>[4x]SIKSEFAEGAAVFVEGVAVFLTMMAAFQNGDKEAVAQYLARGASLYTRHEELLNRLLQKLRREGNKEAVTLMNEFTATFQTGKSLANALIAAFKNGDDDSFESYLQAIWKVIAK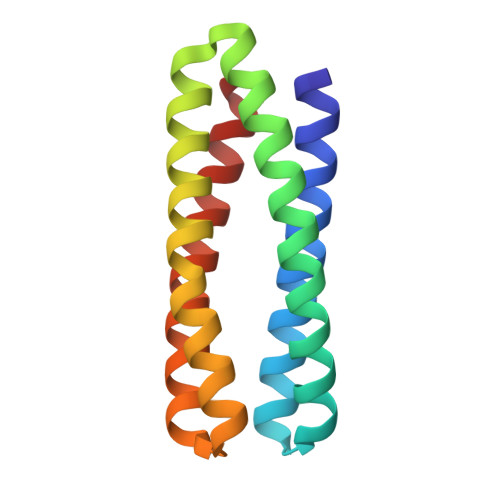MATILDQIAKAI> GHMSFDNYLVPTVIEQSGRGERAFDIYSRLLKERIVFLVGPVTDESANLVVAQLLFLESENPDKDIFFYINSPGGSVTAGMSIYDTMNFIKPDVSTLCLGQAASMGAFLLSAGEKGKRFALPNSRIMIHQ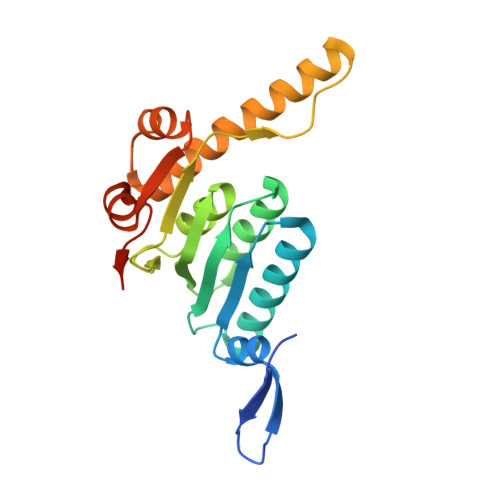PLISGGLGGQASDIEIHARELLKIKEKLNRLMAKHCDRDLADLERDTDRDNFMSAEEAKEYGLIDQILENRASLRL> MASMTGGQQMGRGSMSRDPLPFFPPLYLGGPEITTENCEREPIHIPGSIQPHGALLTADGHSGEVLQMSLNAATFLGQEPTVLRGQTLAALLPEQWPALQAALPPGCPDALQYRATLDWPAAGHLSLTVHRVGELLILEFEPTEAWDSTGPHALRNAMFALESAPNLRALAEVATQTVRELTGFDRVMLYKFAPDATGEVIAEARREGLHAFLGHRFPASDIPAQARALYTR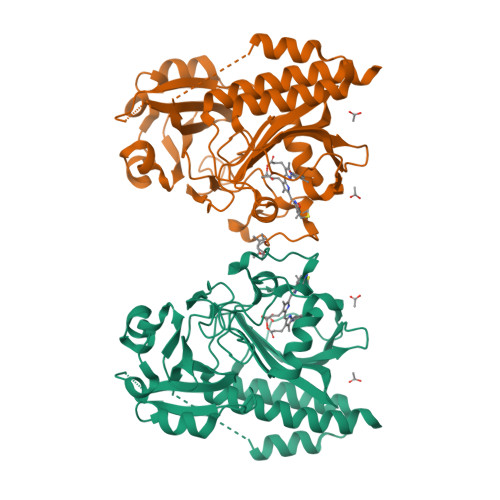HLLRLTADTRAAAVPLDPVLNPQTNAPTPLGGAVLRATSPMHMQYLRNMGVGSSLSVSVVVGGQLWGLIACHHQTPYVLPPDLRTTLEYLGRLLSLQVQVKEALEHHHHHH>[6x]GSHGMGQATAIAHPNIAFIKYWGNRDAVLRIPENGSISMNLAELTVKTTVIFEKHSREDTLILNGALADEPALKRVSHFLDRVREFAGISWHAHVISENNFPTGAGIASSAAAFAALALAATSAIGLHLSERDLSRLARKGSGSACRSIPGGFVEWIPGE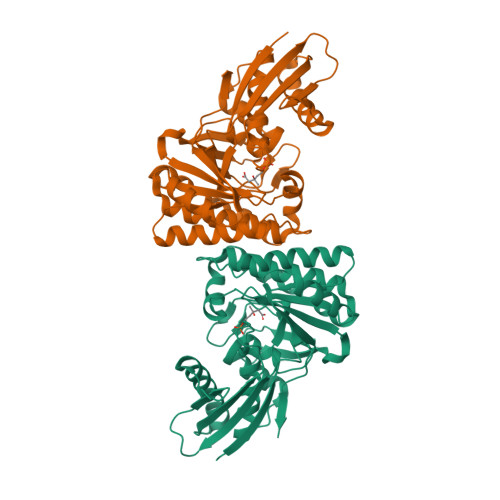TDEDSYAVSIAPPEHWALTDCIAILSTQHKPIGSTQGHALASTSPLQPARVADTPRRLEIVRRAILERDFLSLAEMIEHDSNLMHAVMMTSTPPLFYWEPVSLVIMKSVREWRESGLPCAYTLDAGPNVHVICPSEYAEEVIFRLTSIPGVQTVLKASAGDSAKLIEQSL> DQLDESLRDKVLQLQKGSDTEAQCEVMQEIVDQVLEEDFDSEQLSVLASCLQELFKAHFRGEVLPEEITEESLEESVGKPLYLIFRNLCQMQEDNSSFSLLLDLLSELYQKQPKIGYHLLYYLRASKAAAGKMNLYESFAQATQLGDLHTCLMMDMKACQEDDVRLLCHLTPSIYTEFPDETLRSGELLNMIVAVIDSAQLQELVCHVMMGNLVMFRKDSVLNILIQSLDWETFEQYCAWQLFLAHNIPLETIIPILQHLKYKEHPEALSCLLLQLRREKPSEEMVKMVLSRPCHPDDQFTTSILRHWCMKHDELLAEHIKSLLIKNNSLPRKRQSLRSSSSKLAQLTLEQILEHLDNLRLNLTNTKQNFFSQTPILQALQHVQASCDEAHKMKFSDLFSLAEEYEDSSTKPPKSRRKAALSSPRSRKNATQPPNAEEESGSSSAS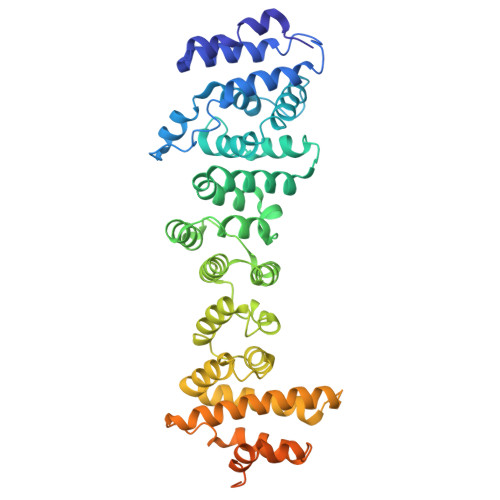EEEDTKPKPTKRKRKGSSAVGSDSD> ETFEHWW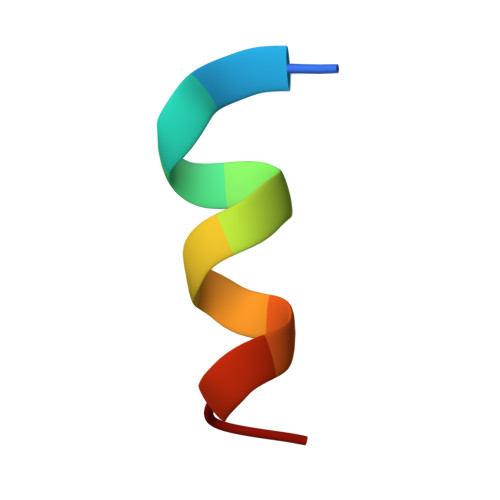SQLLS>[6x]ASTLKSGSKEVENLKKPFMPPREVHVQVTHSMPPQKIEIFKSLDNWAEENI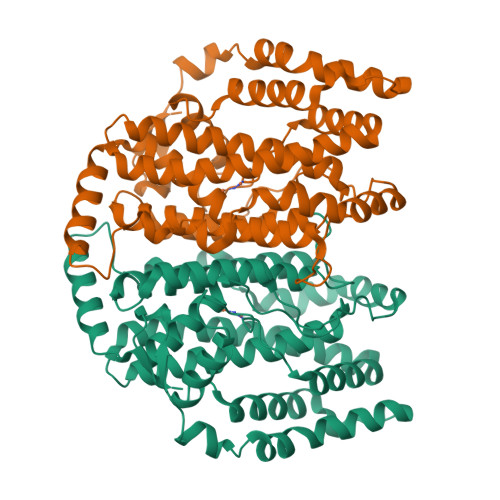LVHLKPVEKCWQPQDFLPDPASDGFDEQVRELRERAKEIPDDYFVVLVGDMITEEALPTYQTMLNTLDGVRDETGASPTSWAIWTRAWTAEENRHGDLLNKYLYLSGRVDMRQIEKTIQYLIGSGMDPRTENSPYLGFIYTSFQERATFISHGNTARQAKEHGDIKLAQICGTIAADEKRHETAYTKIVEKLFEIDPDGTVLAFADMMRKKISMPAHLMYDGRDDNLFDHFSAVAQRLGVYTAKDYADILEFLVGRWKVDKLTGLSAEGQKAQDYVCRLPPRIRRLEERAQGRAKEAPTMPFSWIFDRQVKL>[4x]GAMAAGTLYTYPENWR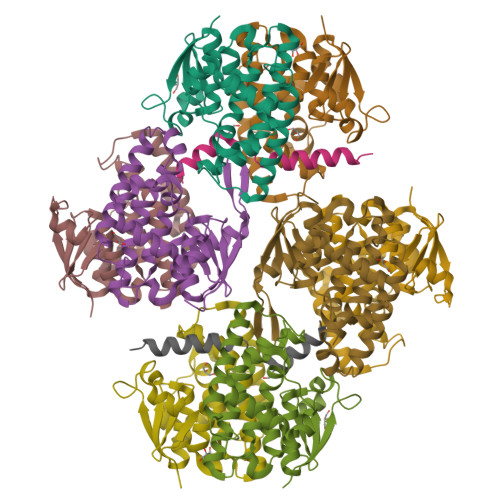AFKALIAAQYSGAQVRVLSAPPHFHFGQTNRTPEFLRKFPAGKVPAFEGDDGFCVFESNAIAYYVSNEELRGSTPEAAAQVVQWVSFADSDIVPPASTWVFPTLGIMHHNKQATENAKEEVRRILGLLDAYLKTRTFLVGERVTLADITVVCTLLWLYKQVLEPSFRQAFPNTNRWFLTCINQPQFRAVLGEVKLCEKMAQFDA;> GAMATNFLAHEKIWFDKFKYDDAERRFYEQMN> PMAAHEASSLYSEEKAKLLREMMAKIEDKNEVLDQFMDSMQLDPETVDNLDAYSHIPPQLMEKCAALSVRPDTVRNLVQSMQVLSGVFTDVEASLKDIRDLLEEDELLEQKFQEAVGQAGAISITSKAELAEVRREWAKYMEVHEKASFTNSELHRAMNLHVGNLRLLSGPLDQVRAALPTPALSPEDKAVLQNLKRILAKVQEMRDQRVSLEQQLRELIQ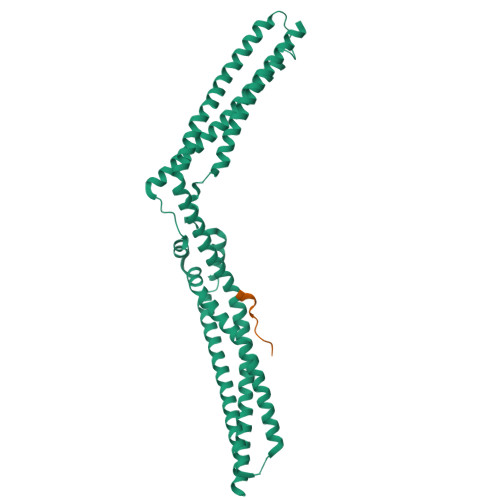KDDITASLVTTDHSEMKKLFEEQLKKYDQLKVYLEQNLAAQDRVLCALTEANVQYAAVRRVLSDLDQKWNSTLQTLVASYEAYEDLMKKSQEGRDFYADLESKVAALLERTQSTCQAREAARQQLLDRELK;> SNIKSLSFPKLDSDDSNQKT>GPVGYGAGTTGGGNKVPVNVATFEAMQSAIDSYSGSGGLVLNYTGKFDFGTIKDVCAQWKLPAKTVQIKNKSDVTIKGANGSAANFGIRVVGNAHNVIIQNMTIGLLQGGEDADSISLEGNSSGEPSKIWVDHNTVFASLTKCSGAGDASFDGGIDMKKGVHHVTVSYNYVYNYQKVALNGYSDSDTKNSAARTTYHHNRFENVESRVPLQRFGLSHIYNNYFNNVTTSGINVRMGGIAKIESNYFENIKNPVTSRDSSEIGYWDLINNYVGSGITWGTPDGSKPYANATNWISTKVFPESLGYIY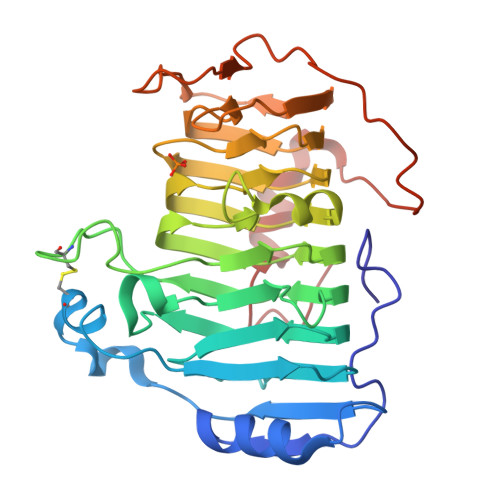TVTPAAQVKAKVIATAGAGKNLAE[2x]>[4x]GSSMDNQDGFILQQVKLSLDDPDSYLSSWNSNDASPCRWSGVSCAGDFSSVTSVDLSSANLAGPFPSVICRLSNLAHLSLYNNSINSTLPLNIAACKSLQTLDLSQNLLTGELPQTLADIPTLVHLDLTGNNFSGDIPASFGKFENLEVLSLVYNLLDGTIPPFLGNI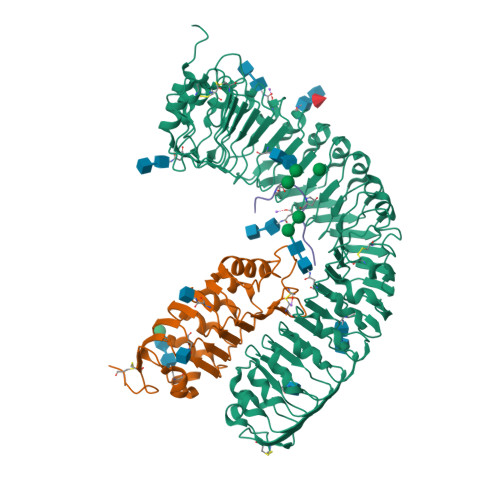STLKMLNLSYNPFSPSRIPPEFGNLTNLEVMWLTECHLVGQIPDSLGQLSKLVDLDLALNDLVGHIPPSLGGLTNVVQIELYNNSLTGEIPPELGNLKSLRLLDASMNQLTGKIPDELCRVPLESLNLYENNLEGELPASIALSPNLYEIRIFGNRLTGGLPKDLGLNSPLRWLDVSENEFSGDLPADLCAKGELEELLIIHNSFSGVIPESLADCRSLTRIRLAYNRFSGSVPTGFWGLPHVNLLELVNNSFSGEISKSIGGASNLSLLILSNNEFTGSLPEEIGSLDNLNQLSASGNKFSGSLPDSLMSLGELGTLDLHGNQFSGELTSGIKSWKKLNELNLADNEFTGKIPDEIGSLSVLNYLDLSGNMFSGKIPVSLQSLKLNQLNLSYNRLSGDLPPSLAKDMYKNSFIGNPGLCGDIKGLCGSENEAKKRGYVLEGSENLYFQ;>[4x]GSSMASANLEGDALHTLRVTLVDPNNVLQSWDPTLVNPCTWFHVTCNNENSVIRVDLGNAELSGHLVPELGVLKNLQYLELYSNNITGPIPSNLGNLTNLVSLDLYLNSFSGPIPESLGKLSKLRFLRLNNNSLTGSIPMSLTNITTLQVLDLSNNRLSGSVPDNGSFSLFTPISFANNLDLCGPVTSHPCPLEGSLENLYFQ;>RLVPSGPNPLHN[4x]>GIVLFVDFDYFYAQVEEVLNPSLKGKPVVVCVFSGRFEDSGAVATANYEARKFGVKAGIPIVEAK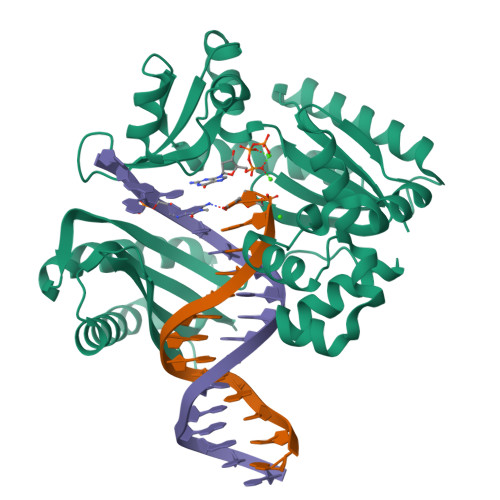KILPNAVYLPMRKEVYQQVSSRIMNLLREYSEKIEIASIDEAYLDISDKVRDYREAYNLGLEIKNKILEKEKITVTVGISKNKVFAKIAADMAKPNGIKVIDDEEVKRLIRELDIADVPGIGNITAEKLKKLGINKLVDTLSIEFDKLKGMIGEAKAKYLISLARDEYNEPIRTRVRKSIGRIVTMKRNSRNLEEIKPYLFRAIEESYYKLDKRIPKAIHVVAVTEDLDIVSRGRTFPHGISKETAYSESVKLLQKILEEDERKIRRIGVRFSKFI[2x]> FRAIIESPEGAGHVGYQYRRNTGSTMRMVSDVLDERVSLWDFHCDPSGNVIQPGPNVDSRQYLQAAIDYVSSNGGGTITIPAGYTWYLGSYGVGGIAGHSGIIQLRSNVNLNIEGRIHLSPFFDLKPFQVFVGFDNGDPASSGNLENCHIYGHGVVDFGGYEFGASSQLRNGVAFGRSYNCSVTGITFQNGDVTWAITLGWNGYGSNCYVRKCRFINLVNSSVNAAHSTVYVNCPYSGVESCYFSMSSSFARNIACSVALH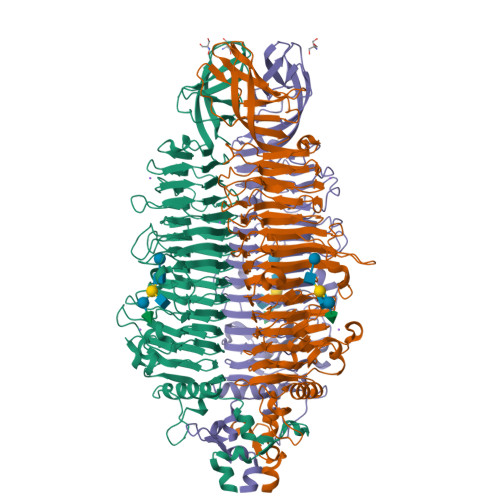QHDTFYRGSTVNGYCRGAYVVMHAAEAAGAGSYAYNMQVENNIAVIYGQFVILGSDVTATVSGHLNDVIVSGNIVSIGERAAFSAPFGAFIDIGPDNSGASNVQDIQRVLVTGNSFYAPANITDSAAITLRANLNGCTFIANNFDCRYMVYNAPGTTSPVVQNLVWDKSNVIGGTHANQRAGQNLFDMQFASVVNSTIEVQLSCEDLSMFSCILFPASCQLSYSKITVDSAWTKSMSNTAVFEGNQQAGANVYVSYPATVNLTSYNTQGAVPFFSTDTNYAWVTSAYSLSINENLDFSPPATYTNKANGQLVGVGYNEIGGVRSVSVRLMLQRQV> MSEEVQERIW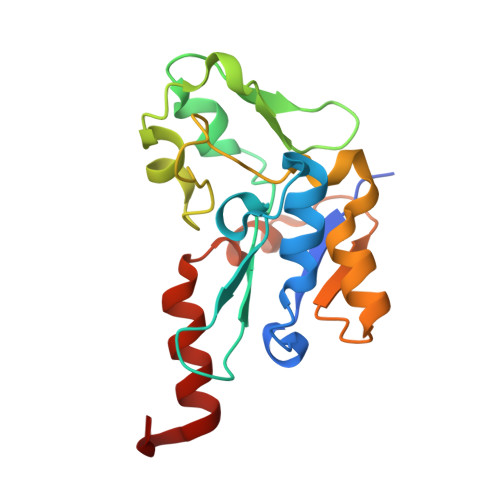ILITPDKCSGCRLCEVTCSLEHEGIIWPEASRIRVFELFPGINVPHTCVQCPDYPCVNACPTNALSVDEKTGAVVVNEEKCITCGACVLACPGKVPRIPAGKGSVVICDLCGGNPKCVEICHEAGHDALKIVTGNYRPIYRTFAKDPQEKSLDIARKVFGEDF>QRCGEQGSNMECPNNLCCSQYGYCGMGGDYCGKGCQNGACWTSKRCGSQAGGATCTNNQCCSQYGYCGFGAEYCGAGCQGGPCRADIKCGSQAGGKLCPNNLCCSQWGFCGLGSEFCGGGCQSGACSTDKPCGKDAGGRVCTNNYCCSKWGSCGIGPGYCGAG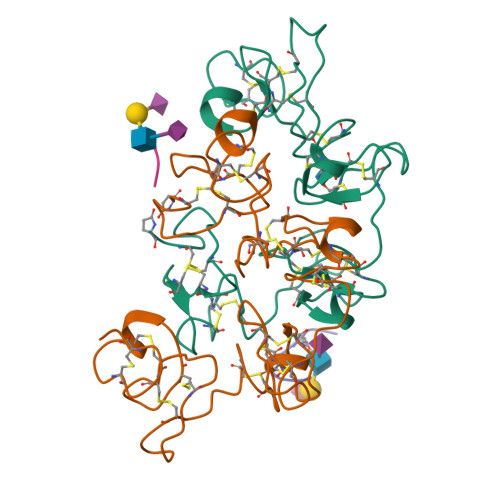CQSGGCDG[2x];>[2x]DTYAATPR> MSKPQPIAAANWKCNGSQQSLSELIDLFNSTSINHDVQCVVASTFVHLAMTKERLSHPKFVIAAQNAGNADGLASLKDFGVNWIVLGHSERRWYYGETNEIVADKVAAAVASGFMVIACIGETLQERESGRTAVVVLTQIAAIAKKLKKADWAKVVIAYEPVWAIGTGKVATPQQAQ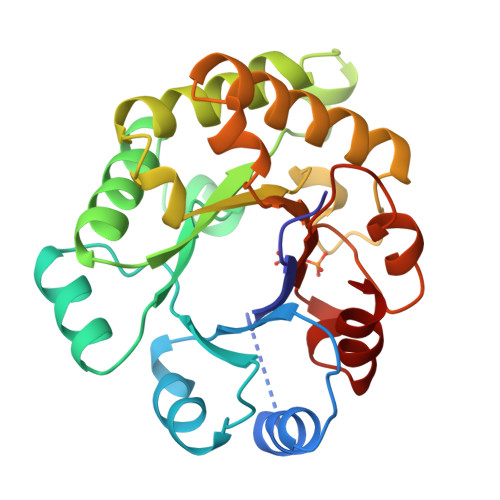EAHALIRSWVSSKIGADVAGELRILYGGSVNGKNARTLYQQRDVNGFLVGGASLKPEFVDIIKATQ(2E,6E)-3,7-dimethyl-8-(phenylamino)octa-2,6-dien-1-yl 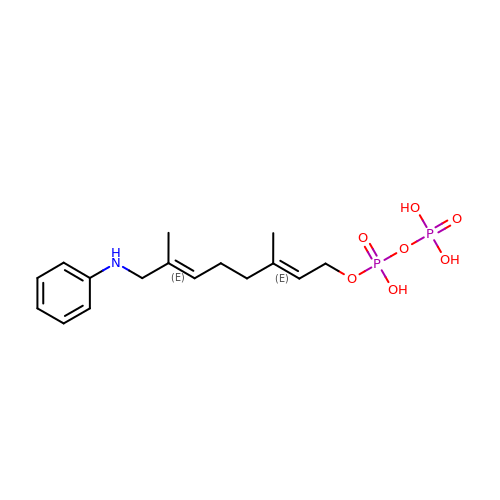trihydrogen diphosphate | C16 H25 N O7 P2 | HODAIPJPJAZJEY-GGQZXFEVSA-N>[3x]MGSSHHHHHHSS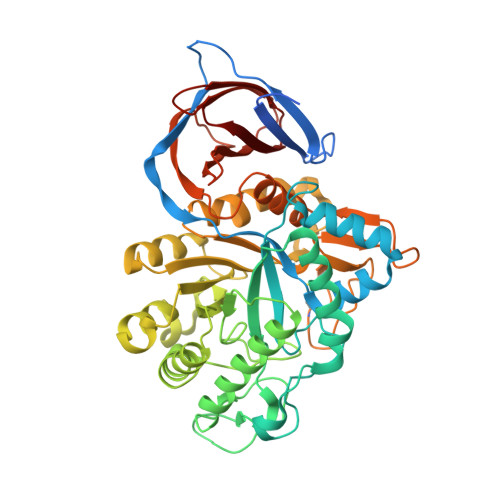GPQQGLRSNSDDAEKPVVPVPTGDVAIYTTTSSLTRDLTRDAVNFSPKDNLAPTTITLNPAEQYQTMDGFGAAITGSTCYNLLLMKPADRHAFLTETFSDKDGFGFSYIRISIGCSDFSLSEYTCCDTKGIENFALQSEEKDYILPILKEILAINPSIKVIAAPWTCPKWMKVKSLTDRTPLDSWTNGQLNPDYYQDYATYFVKWIQAFKAEGIDIYAVTPQNEPLNRGNSASLYMEWEEQRDFVKTALGPQMKAAGLSTKIYAFDHNYNYDNIESQKNYPGKIYEDAAASQYLAGAAYHNYGGNREELLNIHQAYPEKELLFTETSIGTWNSGRDLSKRLMEDMEEVALGTINNWCKGVIVWNLMLDNDRGPNREGGCQTCYGAVDINNSDYKTIIRNSHYYIIAHLSSVVKPGAVRIATTGYTDNGITCSAFENTDGTYAFVLINNNEKSKKITVSDGQRHFAYDVPGKSVTSYRWAKSK>[2x]GPESQLDLRVQELIKLICNVQAMEEMMMEMKYNTKKAPLGKLTVAQIKAGYQSLKKIEDCIRAGQHGRALMEACNEFYTRIPHDFGLRTPPLIRTQKELSEKIQLLEALGDIEIAIKLVKSERQGLEHPLDQHYRNLHCALRPLDHESYEFKVISQYLQSTHAPTHSDYTMTLLDLFEVEKDGEKEAFREDLH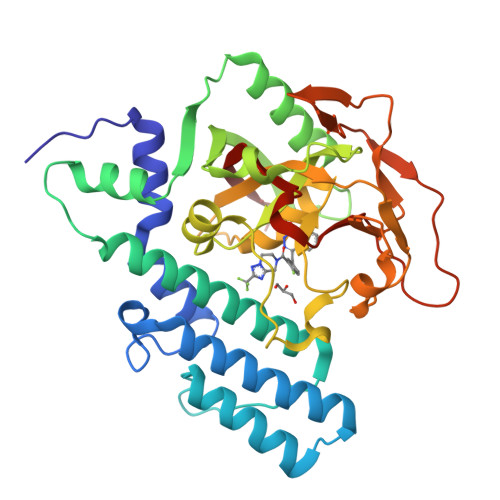NRMLLWHGSRMSNWVGILSHGLRIAPPEAPITGYMFGKGIYFADMSSKSANYCFASRLKNTGLLLLSEVALGQCNELLEANPKAEGLLQGKHSTKGLGKMAPSSAHFVTLNGSTVPLGPASDTGILNPDGYTLNYNEYIVYNPNQVRMRYLLKVQFNFLQ N-[1,1-bis(oxidanylidene)thian-4-yl]-7-(3,4-dimethoxyphenyl)-5-methyl-4-oxidanylidene-thieno[3,2-c]pyridine-2-carboxamide | C22 H24 N2 O6 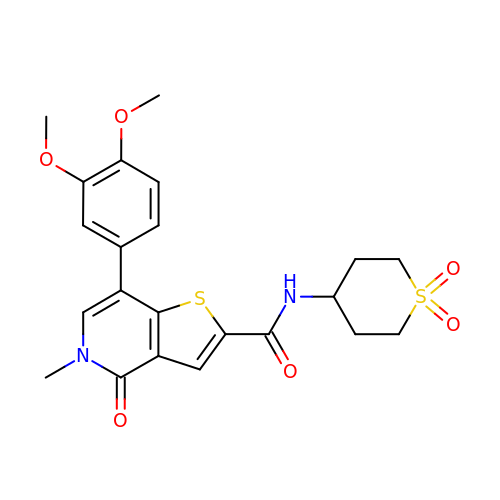S2 | ZJDRXPZROJHILR-UHFFFAOYSA-N> MAEPVENKNQAPAPGAKVPPKGAPAAPKAGAPAAPKGPVAPKAGAPAAKTGASAAKQAGKPRLASLGVTLGRSGVRQESALPYVKPKAVPPPKPAAPAAKGAPAPKGAPAAPAAKAAPGAPVAKAAPKAKKHYFIIENLCVGCGLCLDKCPPKVNAIGYKFYGDVQEGGFRCYIDQAACISCSACFSGDECPSGALIEVLPDGEVLDFSYTPPERLDFDLRFLHRFHREA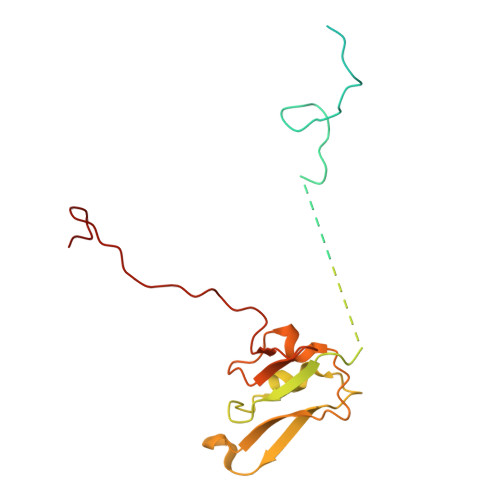R>GSGPAFESYESMELACPAERSGHVAVSDGRHMFVWGGYKSNQVRGLYDFYLPREELWIYNMETGRWKKINTEGDVPPSMSGSCAVCVDRVLYLFGGHHSRGNTNKFYMLDSRSTDRVLQWERIDCQGIPPSSKDKLGVWVYKNKLIFFGG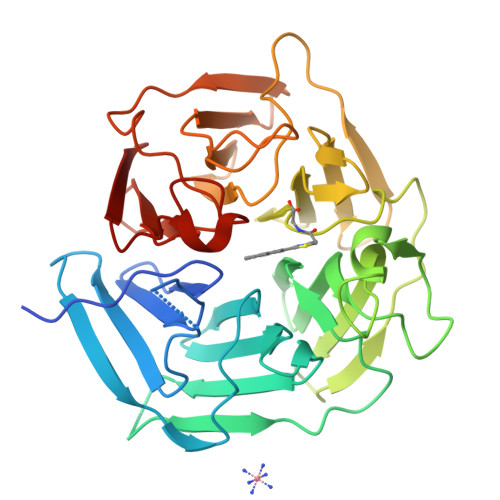YGYLPEDKVLGTFEFDETSFWNSSHPRGWNDHVHILDTETFTWSQPITTGKAPSPRAAHACATVGNRGFVFGGRYRDARMNDLHYLNLDTWEWNELIPQGICPVGRSWHSLTPVSSDHLFLFGGFTTDKQPLSDAWTYCISKNEWIQFNHPYTEKPRLWHTACASDEGEVIVFGGCANNLLVHHRAAHSNEILIFSVQP[2x]>MANELTWHDVLAEEKQQPYFLNT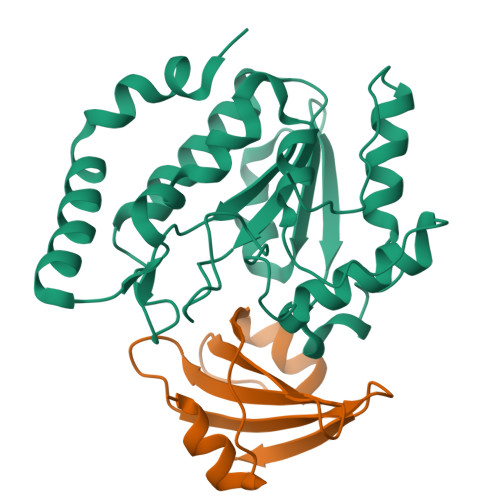LQTVASERQSGVTIYPPQKDVFNAFRFTELGDVKVVILGQDPYHGPGQAHGLAFSVRPGIAIPPSLLNMYKELENTIPGFTRPNHGYLESWARQGVLLLNTVLTVRAGQAHSHASLGWETFTDKVISLINQHREGVVFLLWGSHAQKKGAIIDKQRHHVLKAPHPSPLSAHRGFFGCNHFVLANQWLEQRGETPIDWMPVLPAESE[4x];>[4x]MTNLSDIIEKETGKQLVIQESILMLPEEVEEVIGNKPESDILVHTAYDESTDENVMLLTSDAPEYKPWALVIQDSNGENKIKML>MTTITTYPGVYIEEDASLSLSVSSSATAVPVFAVAGDNPLISGKPYIRISNWLEYLTLKNEQFDPANTLDISLRAYFINGGGYCYLVQTTDLEKQVPKLDDVTLLVAAGENITTAVSTLCKPGKGLFAIFDGPTTELKSDGTSNSDYDPNPFAAVYYPWLTADWTTTIDIPPSAAIAGVYCSVDSTRGVWKAPANVPIQGGLQPKYPVTDDLQAQYNQGKALNMIRTFPKSGTLVWGARTLEDNDNWRYIPVRRLFNSAERDIKNAMSFAVFEPNSQPTWERVRSAVNNYLYSLWQQGGLAGNKPDDAYFVQIGKDITMTDDDIKQGKMIIKIGMAAVRPAEFIILQFTQNTAQ[12x];>[6x]MPTIPTYPGVYIEEDASLNLSVNQGNTAIPVFIGLFSPKNTNLKSQVTRVNSWLDFTNLFNAGCIAPITIKSTKRASMPAPTLLENVKGDTAVVATPGISVDADNKDPTYTYKVIVNYTTSSDALKLYFQNGGGPCYILPQLDRLTQGFLDSIPELIKQALEITLIVCPEWDSGYQSKIYNSLTSSLLNAGYFLIADNQDKNTALITEVASQTATYYPAVKVSQLIQAEDSQIAVSGYEDAKTKSDEVKNLAQLKEKNPTVYQQAVQKIQAIQDEIAANGNIIPVSAVMAGIYCATDASRGVWKAPANIVLSGISDVAERLTDDEQGEMNSKGINAIRYFSHKGFVVWGARTLQNDDNWRYIPVRRLFNAAERDIKQAMQSVVFEPNSQPTWERVKSAIDNYLYSLWQQGALAGNKPQEAYFVQIGKDVTMSDDDIKQGKMI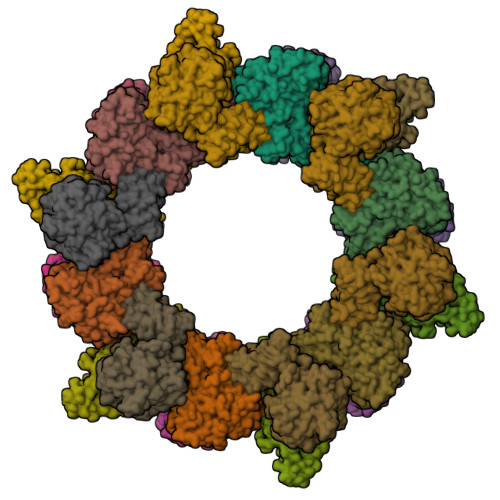VKVGMAAVRPAEFIILQFSQQVAQ;>MEITQPSVTITENLIFPKQNDSFIGIPVFIGYTSSPVDKTAIKLHSLADFARSFPESGLMYYSVRHFFENGGQQAYVLSLGTEQQLSDFSSLITALQQAWLAQTIAAENDITLIITPDVIRFDQTEISDTQRDLWLQLWQSVLNLCKSRRGIMGLLDAPDDPTLAAKCLQQFSSADRQWGVVYWPLLKSAYQDNTQNPIVLSPTAAVAAVIQRNDNQQGVWTAPANIALSKVISPVRAYIEANALFNPDGTSLNLVRSFPGKGIRIWGCRTLENTHDSPWSYIQTRRLVSYIEAYMTQLGRAFVFEPNNAITWMKFKGQAHNWLRQLWLKGGLRGTQEDQAFEVLLGVDESMREADLRAGKMIIKIRLAVLIPAEFIELNLTFDTRTGTIPS[6x]> MGSSHHHHHHSSGLVPAGSHMEFAQHPLTPNGRKAGSAGDTALAFWKDHLSWWHDWTPAPSSPKGAGLVPVSMLWGGGNNGQKDAQRLQQFEHLNSTPAYVMGFNEPDCSGADVSADIDVNTGVSLWNSLIAPMGQ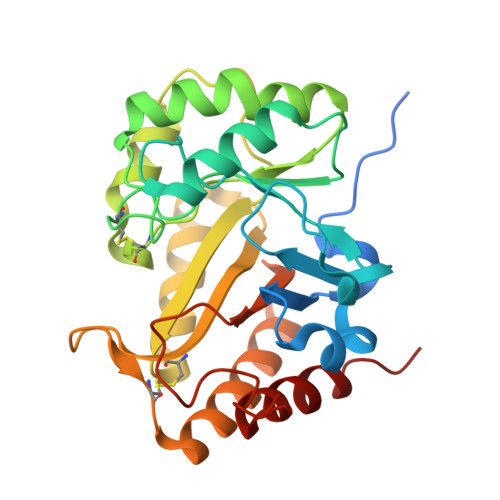KGAALGSPAMCRQKDESWLKQFNQQQLTKSWDFTSIHIFKSDMTGVQADIDYYWNTYQKPLWVTEFACVFDQNNFTPCTDQNQINQWISDIVDLFEANEHVLAYAYTDGLGLGSVWPPVNSDGSLSQSGQAYLNAISKYHSR> GSHMKYHVGIDVGTFSVGLAAIEVDDAGMPIKTLSLVSHIHDSGLDPDEIKSAVTRLASSGIARRTRRLYRRKRRRLQQLDKFIQRQGWPVIELEDYSDPLYPWKVRAELAASYIADEKERGEKLSVALRHIARHRGWRNPYAKVSSLYLPDGPSDAFKAIREEIKRASGQPVPETATVGQMVTLCELGTLKLRGEGGVLSARLQQSDYAREIQEICRMQEIGQE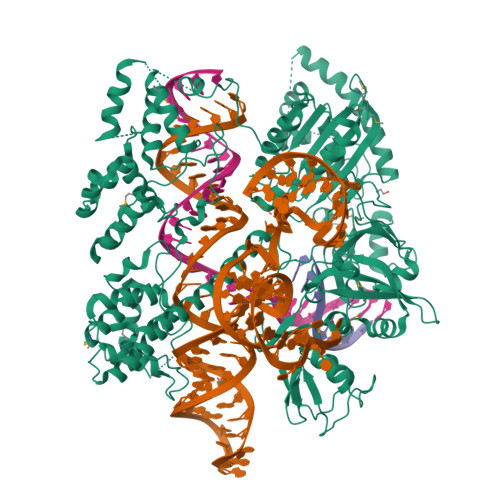LYRKIIDVVFAAESPKGSASSRVGKDPLQPGKNRALKASDAFQRYRIAALIGNLRVRVDGEKRILSVEEKNLVFDHLVNLTPKKEPEWVTIAEILGIDRGQLIGTATMTDDGERAGARPPTHDTNRSIVNSRIAPLVDWWKTASALEQHAMVKALSNAEVDDFDSPEGAKVQAFFADLDDDVHAKLDSLHLPVGRAAYSEDTLVRLTRRMLSDGVDLYTARLQEFGIEPSWTPPTPRIGEPVGNPAVDRVLKTVSRWLESATKTWGAPERVIIEHGGGSGGSMESVAWMANELRSRVAQHFASHGTTVRVYRGSLTAEARRASGISGKLKFFDGVGKSRLDRRHHAIDAAVIAFTSDYVAETLAVRSNLKQSQAHRQEAPQWREFTGKDAEHRAAWRVWCQKMEKLSALLTEDLRDDRVVVMSNVRLRLGNGSAHKETIGKLSKVKLSSQLSVSDIDKASSEALWCALTREPGFDPKEGLPANPERHIRVNGTHVYAGDNIGLFPVSAGSIALRGGYAELGSSFHHARVYKITSGKKPAFAMLRVYTIDLLPYRNQDLFSVELKPQTMSMRQAEKKLRDALATGNAEYLGWLVVDDELVVDTSKIATDQVKAVEAELGTIRRWRVDGFFSPSKLRLRPLQMSKEGIKKESAPELSKIIDRPGWLPAVNKLFSDGNVTVVRRDSLGRVRLESTAHLPVTWKVQ>SMRKSREYEHVRRDLDPNEVWEIVGELG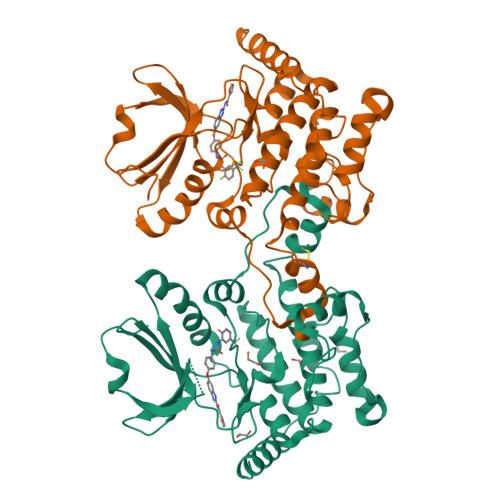DGAFGKVYKAKNKETGALAAAKVIETKSEEELEDYIVEIEILATCDHPYIVKLLGAYYHDGKLWIMIEFCPGGAVDAIMLELDRGLTEPQIQVVCRQMLEALNFLHSKRIIHRDLKAGNVLMTLEGDIRLADFGVSAKNLKTLQKRDSFIGTPYWMAPEVVMCETMKDTPYDYKADIWSLGITLIEMAQIEPPHHELNPMRVLLAIAASDPPTLLTPSKWSVEFRDFLAIALDKNPETRPSAAQLLEHPFVSSITSNKALRELVAEAKAEVMEE[2x]As an important member, 4-hydroxyphenylpyruvate dioxygenase (HPPD) catalyzes the complex transformation of 4-hydroxyphenylpyruvate acid (HPPA) to homogentisic acid (HGA), a key step in the tyrosine catabolic pathway that is common to all the aerobic organisms. In plants, HGA is a key intermediate in the biosynthesis of tocopherols and plastoquinones, which are essential compounds for the photosynthesis. Inhibition of the enzyme results in foliage bleaching of plants and eventually death, and thus HPPD inhibitors have been developed as herbicides for many years. Each monomeric unit consists of nine α-helices and sixteen β-strands that form two barrel-shaped structural domains: a conserved C-terminal domain containing the active site and a diversified N-terminal loop domain.

Inhibitory kinetic analysis towards the recombinant AtHPPD indicated that Y13161 is a competitive inhibitor (Ki = 24.16 ± 1.01 nM) with respect to HPPA with the characteristic of slow binding (and). Similar to all the known inhibitors, two carbonyl groups on Y13161 formed clear chelation interaction between its two carbonyl groups with the metal ion and a pronounced π-π stacking interaction between quinazoline-2,4-dione moiety and two aromatic residues (Phe381 and Phe424) (, and). Additionally, the cyclohexane moiety interacts with the surrounding hydrophobic residues like Phe419, Pro280, Val269, and Val228. Intriguingly, the benzene ring at the N-1 position of the quinazoline-2,4-dione ring formed π-π stacking interaction with Phe392, which results in the more complementary in shape to HPPD active site. It should be pointed out that the interaction with Phe392 has never been observed before in other HPPD inhibitor complexes. Most importantly, the conformation of the active site of AtHPPD-Y13161 overlaps very well with that of the holo-AtHPPD, but remarkably different from that of AtHPPD-HPPA complex, suggesting that the binding of Y13161 indeed keep HPPD in inactive state as expected. As a consequence, the H-bond network of Ser267-Asn282-Gln307-Gln293 would not form due to the far distance (~5.0 Å) between Gln293 and Gln307. On the contrary, the H-bond network of Glu394-Gln379-Asn423 appears around the Y13161, just like its presence in the active site of holo-AtHPPD structure. Collectively, these observations confirmed solidly that targeting the conformational change of Gln293 is an effective way to design new HPPD inhibitors. Overall, due to its excellent herbicidal activity, crop safety, and toxicological properties, Y13161 (the approved common name is Benquitrione) has progressed into industry development and will get registration as a selective herbicide for the weed control in sorghum field from the Institute for the Control of Agrochemicals, Ministry of Agriculture (ICAMA) of China.

> MFVRKNPKSDKFKVKRFHHIEFWCGDATNVARRFSWGLGMRFSAKSDLSTGNMVHASYLLTSGDLRFLFTAPYSPSLSAGEIKPTTTASIPSFDHGSCRSFFSSHGLGVRAVAIEVEDAESAFSISVANGAIPSSPPIVLNEAVTIAEVKLYGDVVLRYVSYKAEDTEKSEFLPGFERVEDASSFPLDYGIRRLDHAVGNVPELGPALTYVAGFTGFHQFAEFTADDVGTAESGLNSAVLASNDEMVLLPINEPVHGTKRKSQIQTYLEHNEGAGLQHLALMSEDIFRTLREMRKRSSIGGFDFMPSPPPTYYQNLKKRVGDVLSDDQIKECEELGILVDRDDQGTLLQIFTKPLGDRPTIFIEIIQRVGCMMKDEEGKAYQSGGCGGFGKGNFSELFKSIEEYEKTLEAKQLVG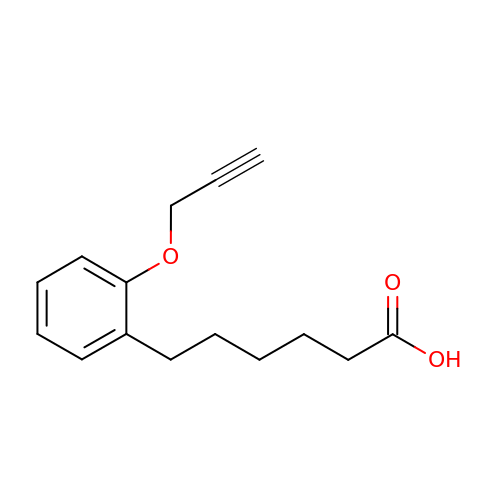6-(2-prop-2-ynoxyphenyl)hexanoic acid | C15 H18 O3 | CUNYTKVXYZYERK-UHFFFAOYSA-N>MRRSVYLDNTIEFLRGRVYLGAYDYTPEDTDELVFFTVEDAIFYNSFHLDFGPMNIGHLYRFAVIFHEILNDPENANKAVVFYSSASTRQRANAACMLCCYMILVQAWTPHQVLQPLAQVDPPFMPFRDAGYSNADFEITIQDVVYGVWRAKEKGLIDLHSFNLESYEKYEHVEFGDFNVLTPDFIAFASPQEDHPKGYLATKSSHLNQPFKSVLNFFANNNVQLVVRLNSHLYNKKHFEDIGIQHLDLIFEDGTCPDLSIVKNFVGAAETIIKRGGKIAVHCKAGLGRTGCLIGAHLIYTYGFTANECIGFLRFIRPGMVVGPQQHWLYLHQNDFREWKYTTRISLKPSEAIGGLYPLISLEEYRLQKKKLKD[2x];> AFTDVPALNYPATPPP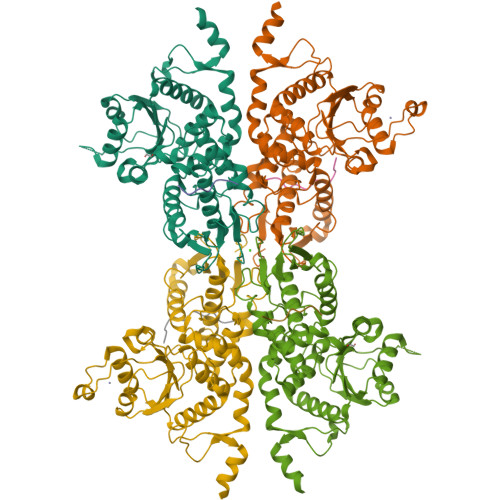H;> FTDVPALNYPATPPPH> GPHMGAYWMSPTADDIRAMNRMQRQRVVGFTVGRENVGSVQFKVPVDLSNINLDDLFGTIVILEPRSATVYPNAAKKPPMGK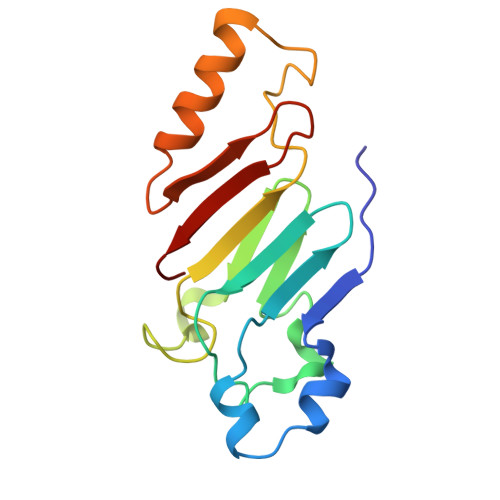GLNVPALISLEHSWPRGGPTIKGRRLERHIERLKSIPDTTFESYDPETGVWAFSVEHF>[4x]DHYN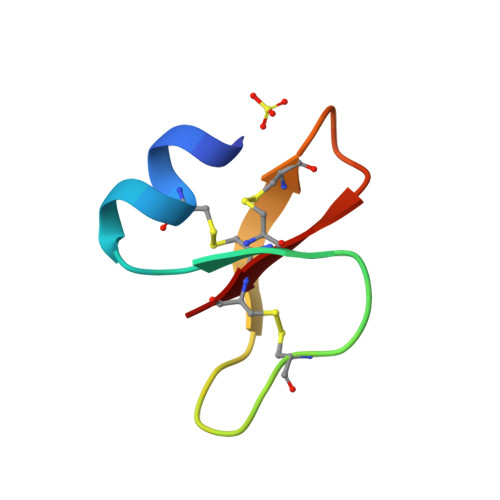CVSSGGQCLYSACPIFTEIQGTCYRGKAKCCK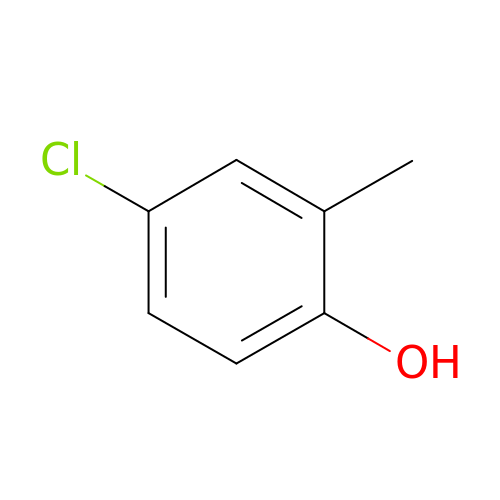4-chloro-2-methylphenol | C7 H7 Cl O | RHPUJHQBPORFGV-UHFFFAOYSA-N>KKGFEFTLM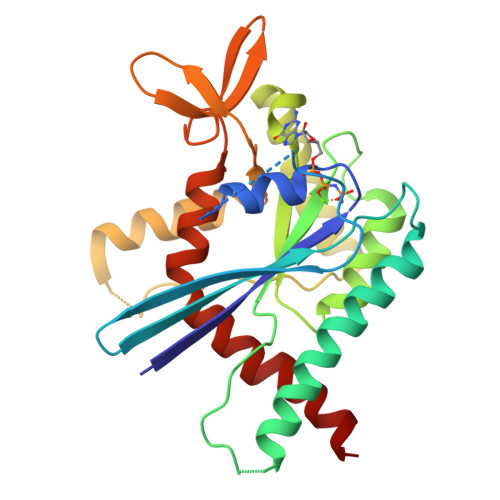VVGESGLGKSTLINSLFLTDLYPERIIPGAAEKIERTVQIEASTVEIEERGVKLRLTVVDTPGYGDAINCRDCFKTIISYIDEQFERYLHDESGLNRRHIIDNRVHCCFYFISPFGHGLKPLDVAFMKAIHNKVNIVPVIAKADTLTLKERERLKKRILDEIEEHSIKIYHLPDAESDEDEDFKEQTRLLKASIPFSVVGSNQLIEAKGKKVRGRLYPWGVVEVENPEHNDFLKLRTMLITHMQDLQEVTQDLHYENFRSERLKR[4x]> MHHHHHHHHGSENLYFQGSGSTQLQLHGLLSNISSKEGTYAKLGGLYTQSLARLVAKCEDLFMGGQKKELHFNENNWSLFKLTCNKPCCDSGDAIYYCATCSEDPGSTYAVKICKAPEPKTVSYCSPSVPVHFNIQQDCGHFVASVPSSMLSSPDAPKDPVPALPTHPPAQEQDCVVVITREVPHQTASDFVRDSAASHQAEPEAYERRVCFLLLQLCNGLEHLKEHGIIHRDLCLENLLLVHCTLQAGPGPAPAPAPAPAAAAPPCSSAAPPAGGTLSPAAGPASPEGPREKQLPRLIISNFLKAKQKPGGTPNLQQKKSQARLAPEIVSASQYRKFDEFQTGILIYELLHQPNPFEVRAQLRERDYRQEDLPPLPA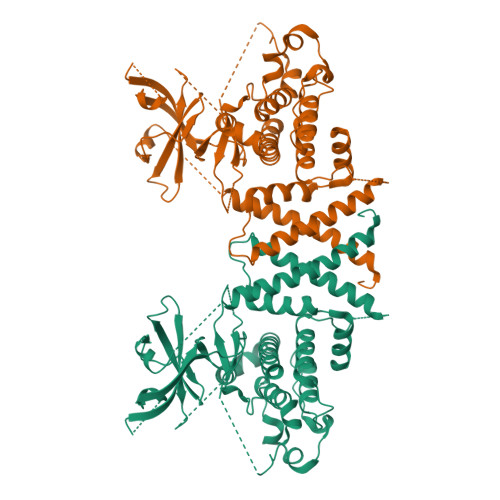LSLYSPGLQQLAHLLLEADPIKRIRIGEAKRVLQCLLWGPRRELVQQPGTSEEALCGTLHNWIDMKRALMMMKFAEKAVDRRRGVELEDWLCCQYLASAEPGALLQSLKLLQLL> MNQVQRSNELSQERTARLNELQRALVMMDSDFRQIALRQTRTNGEEPSKKLLHWADYLLDSDNKGIMFARLGWHNPQQQFPRGEVTKVGYRIKDERLERVWWRYPDTPAGQEGVVTPLLSDVEELNVRFYDGKQWINEWSNELTLPAAISV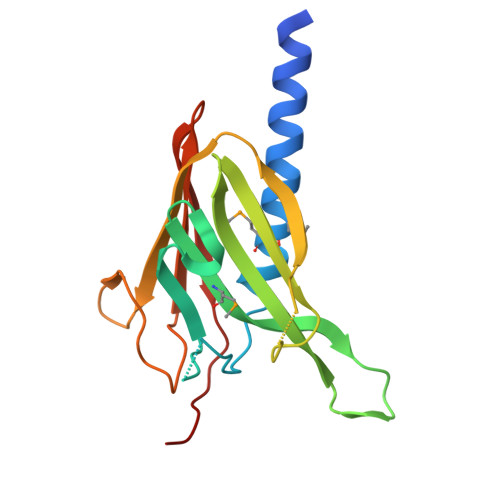ELTLKDYGKIARTYLTPEGNLQKQ> ACGTCA;> GAACGACAGTGACGTCGACTC;>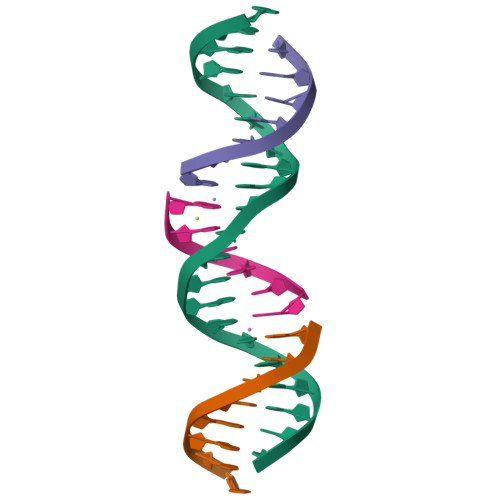 TCGAGTCG;> CTGTCGT>[4x]MTNIEPVIIETRLELIGRYLDHLKKFENISLDDYLSSFEQQLITERLLQLITQAAIDINDHILS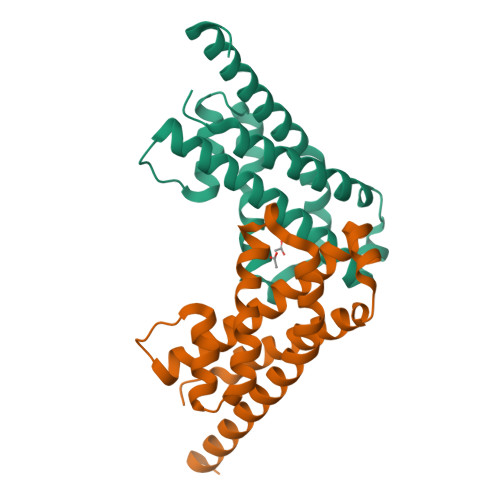KLKSGKSYTNFEAFIELGKYQILTPELAKQIAPSSGLANRLVHEYDDIDPNQVFMAISFALQQYPLYVRQINSYLITLEEENDLESGHHHHHH>[2x]NPCIEVVPNITYQCMDQKLSKVPDDIPSSTKNIDLSFNPLKILKSYSFSNFSELQWLDLSRCEIETIEDKAWHGLHHLSNLILTGNPIQSFSPGSFSGLTSLENLVAVETKLASLESFPIGQLITLKKLNVAHNFIHSCKLPAYFSNLTNLVHVDLSYNYIQTITVNDLQFLRENPQVNLSLDMSLNPIDFIQDQAFQGIKLHELTLRGNFNSSNIMKTCLQNLAGLHVHRLILGEFKDERNLEIFEPSIMEGLCDVTIDEFRLTYTNDFSDDIVKFHCLANVSAMSLAGVSIKYLEDVPKHFKWQSLSIIRCQLKQFPTLDLPFLKSLTLTMNKGSISFKKVALPSL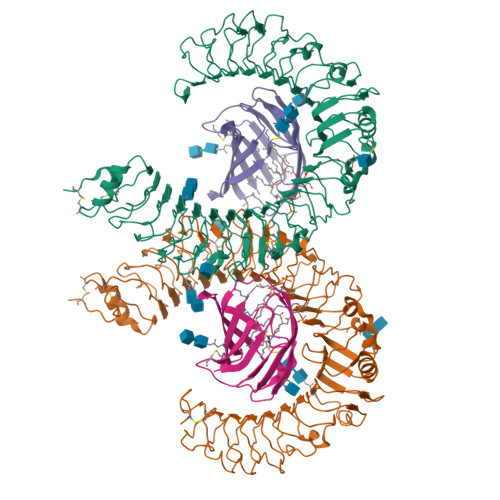SYLDLSRNALSFSGCCSYSDLGTNSLRHLDLSFNGAIIMSANFMGLEELQHLDFQHSTLKRVTEFSAFLSLEKLLYLDISYTNTKIDFDGIFLGLTSLNTLKMAGNSFKDNTLSNVFANTTNLTFLDLSKCQLEQISWGVFDTLHRLQLLNMSHNNLLFLDSSHYNQLYSLKELALDTNQLKSVPDGIFDRLTSLQKIWLHTNPWDCSCPRIDYLSRWLNKNSQKEQGSAKCSGSGKPVRSIICPT;>EKQQWFCNSSDAIISYSYCDHLKFPISISSEPCIRLRGTNGFVHVEFIPRGNLKYLYFNLFISVNSIELPKRKEVLCHGHDDDYSFCRALKGETVNTSIPFSFEGILFPKGHYRCVAEAIAGDTEEKLFCLNFTIIHRRDVNKGENLYFQ[2x]> M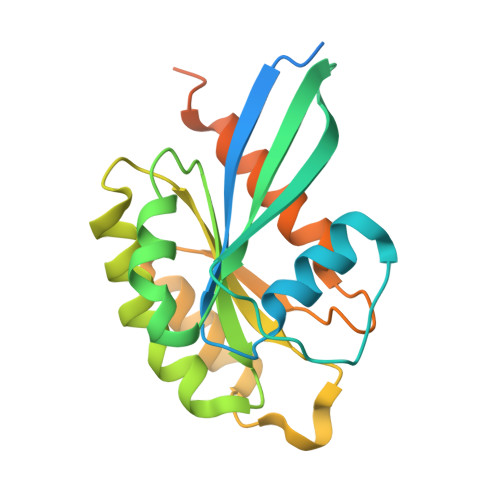AHHHHHHSSGASAQDARYGQKDSSDQNFDYMFKLLIIGNSSVGKTSFLFRYADDSFTSAFVSTVGIDFKVKTVFKNEKRIKLQIWDTAGQERYRTITTAYYRGAMGFILMYDITNEESFNAVQDWSTQIKTYSWDNAQVILVGNKCDMEDERVISTERGQHLGEQLGFEFFETSAKDNINVKQTFERLVDIICDKMSESLETDPAITAAKQNTRLKETPPPPHPNCGC> GPHMSLSVAEKSYLYDSLASTPSIRPDGRLPHQFRPIEIFTDFLPSSNGSSRIIASDGSECIVSIKSKVVDHHVENELLQVDVDIAGQRDDALVVETITSLLNKVLKSGSGVDSSKLQLTKKYSFKIFVDVLVISSHSHPISLISFAIYSA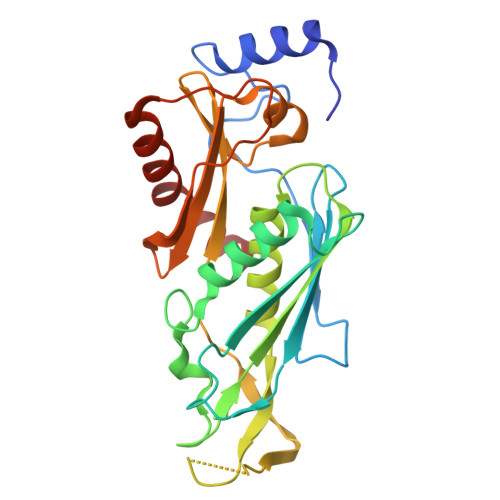LNSTYLPKLISAFDDLEVEELPTFHDYDMVKLDINPPLVFILAVVGNNMLLDPAANESEVANNGLIISWSNGKITSPIRSVALNDSNVKSFKPHLLKQGLAMVEKYAPDVVRSLENL>GPQPLPSAPENNPEEELASKQKNEESKKRQWALEDFEIGRPLGKGKFGNVYLAREKQSKFILALKVLFKAQLEKAGVEHQLRREVEIQSHLRHPNILRLYGYFHDATRVYLILEYAPLGTVYRELQKLSKFDEQRTATYITELANALSYCHSKRVIHRDIKPENLLLGSA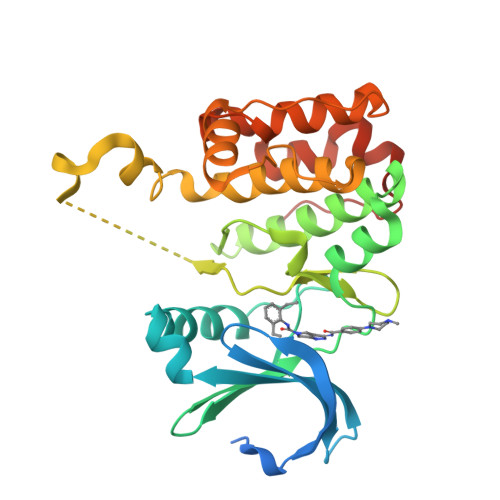GELKIADFGWSVHAPSSRRDDLCGTLDYLPPEMIEGRMHDEKVDLWSLGVLCYEFLVGKPPFEANTYQETYKRISRVEFTFPDFVTEGARDLISRLLKHNPSQRPMLREVLEHPWITANSSKPSNCQNKESASKQS[6x]>MKKLYTSYG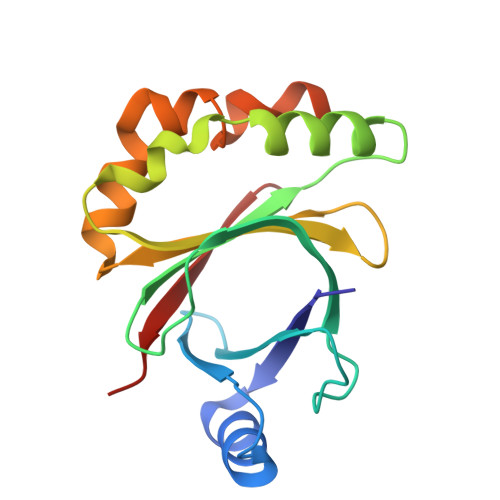TYGFLHQIKINNPTHQLFQFSASDTSVIFEETDGETVLKSPSIYEVIKEIGEFSEHHFYCAIFIPSTEDHAYQLEKKLISVDDNFRNFGGFKSYRLLRPAKGTTYKIYFGFADRHAYEDFKQSDAFNDHFSKDALSHYFGSSGQHSSYFERYLYPIKE[4x]> GQEREAAEYIAQARRQYHFESNQRTCNMTVLSMLPTLREALMQQLNSESLTALLKNRPSNKLEIWEDLKIISFTRSTVAVYSTCMLVVLLRVQLNIIGGYIYLDNAAVGKNGTTILAPPDVQQQYLSSIQHLLGDGLTELITVIKQAVQKVLGSVSLKHSLSLLDLEQKLKEIRNLVEQHKSSSWINKDGSKPLLSHYMMPDEETPLAVQ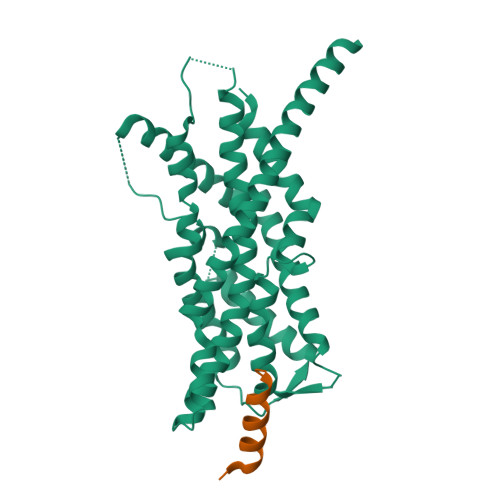ACGLSPRDITTIKLLNETRDMLESPDFSTVLNTCLNRGFSRLLDNMAEFFRPTEQDLQHGNSMNSLSSVSLPLAKIIPIVNGQIHSVCSETPSHFVQDLLTMEQVKDFAANVYEAFSTPQQLEK;> ADRELEELLESALDDFDKAK(2S,3R)-2-[[2-methyl-3-oxidanyl-5-(phosphonooxymethyl)pyridin-4-yl]methylamino]-3-oxidanyl-pentanoic 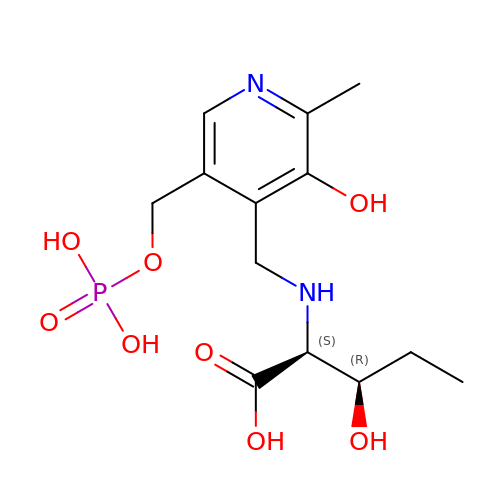acid | C13 H21 N2 O8 P | BXUMTZWSUSTQMU-MNOVXSKESA-N> 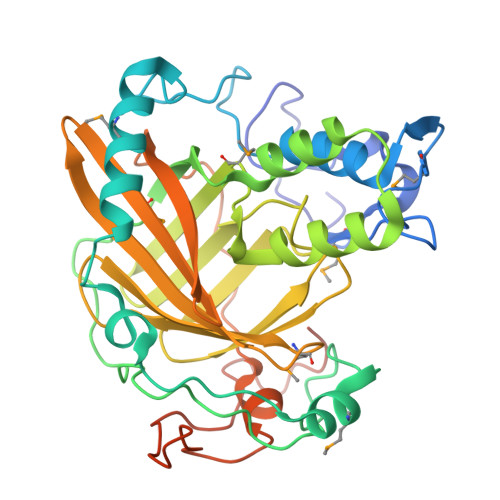VCEKGFEAGDNKLGGALNAKHVEKYGDNFKNGMHKPEFHEDGLHKPMEVGGKKFESGFHYLLECHELGGKNASGGYGGPLCEDPYGSEVQAMTEKLLKEADSDRTLCFNNFQDPCPQLTKEQVAMCKGFDYGDKTLKLPCGPLPWPAGLPEPGYVPKTNPLHGRWITVSGGQAAFIKEAIKSGMLGAAEANKIVADTDHHQTGGMYLRINQFGDVCTVDASVAKFARAKRTWKSGHYFYEPLVSGGNLLGVWVLPEEYRKIGFFWEMESGRCFRIERRAFPVGPYTFMRQATEVGGKISFVFYVKVSNDPESDPIPLQSRDYTALAGRDNAPTNLGKPYPTLAKDLDYPKKRDGWLEKNEKEMLRQRNIVSSTF> MRSRRVDVMDVMNRLILAMDLMNRDDALRVTGEVREYIDTVKIGYPLVLSEGMDIIAEFRKRFGCRIIADFAVADIPETNEKICRATFKAGADAIIVHGFPGADSVRACLNVAEEMGREVFLLTEMSHPGAEMFIQGAADEIARMGVDLGVKNYVGPSTRPERLSRLREIIGQDSFLISPGVGAQGGDPGETLRFADAIIVGRSIYLADNPAAAAAGIIESIKDLLIPEDPAANKARK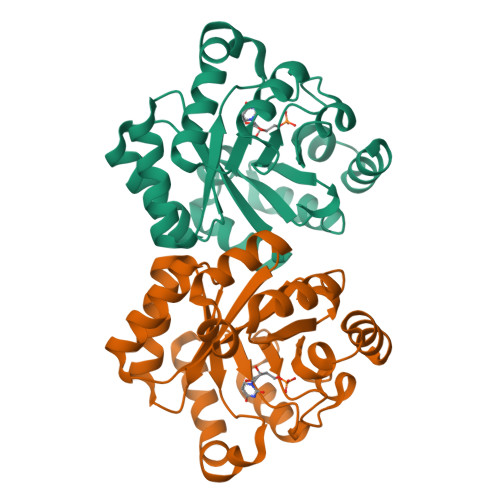EAELAAATA GALANTHAMINE DERIVATIVE | C32 H37 N2 O5 | 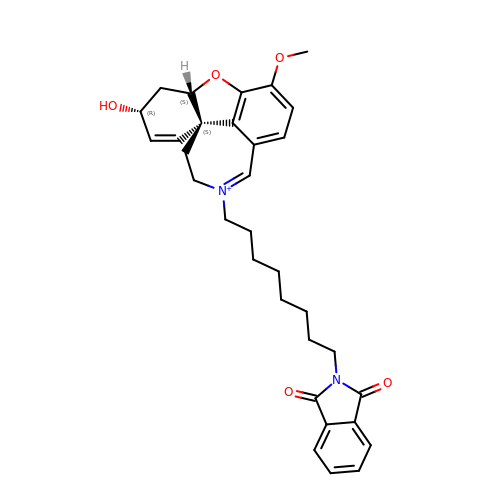VLGAHTYYCHWLNI-BHRZLAGCSA-N>[8x]MLTEFDAGYGEQPFRDLCANYPGAEAYDPHDFRIEWGPIFHRGRLDGSARVLIVGQDPAQHETIVRRILVGTAGRRTQGFLAK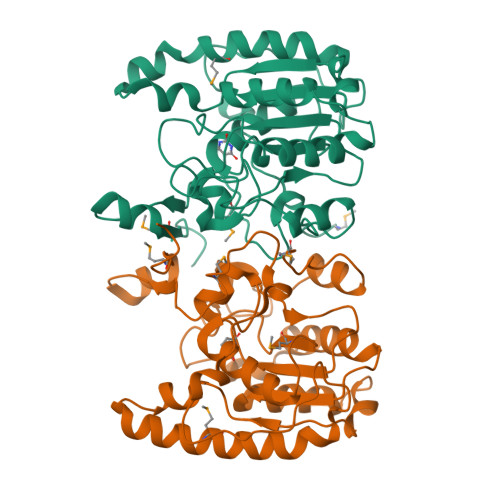LGIVQSYVMVNTFLYSVYGQSGGSKHKNEPGIVDYRNKWFKAVLGPGNIEAVVSLGGLADEAWKAWLKSSDGAAYKTLAYQHITHPTWPESSAHDSATQAANTKIMLAKWNAALAALAPEVKHPDVPTTLVPYGDAFKPSELVDIIAKDLPAGLPAWMRGDTPWAVRQGVDAAAKRRTIMITIPDGVIP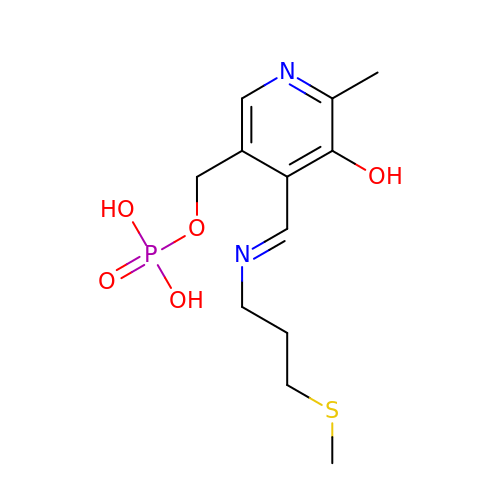[6-methyl-4-[(E)-3-methylsulfanylpropyliminomethyl]-5-oxidanyl-pyridin-3-yl]methyl dihydrogen phosphate | C12 H19 N2 O5 P S | BEOXZSCYUHRCGB-NTUHNPAUSA-N> QNSETGALKTFITQQGIKSQHQTKEEQSQITSQVTGQIGWRREGIKYRRNELFLDVLESVNLLMSPQGQVLSAHVSGRVVMKSYLSGMPECKFGMNDKIVIEKQGKGTADETSKSGKQSIAIDDCTFHQCVRLSKFDSERSISFIPPDGEFELMRYRTTKDIILPFRVI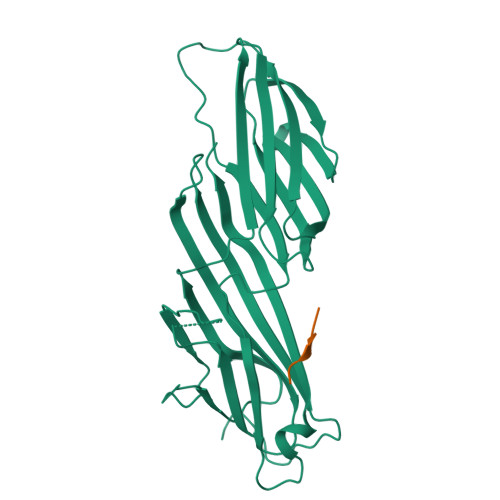PLVREVGRTKLEVKVVIKSNFKPSLLAQKIEVRIPTPLNTSGVQVICMKGKAKYKASENAIVWKIKRMAGMKESQISAEIELLPTNDKKKWARPPISMNFEVPFAPSGLKVRYLKVFEPKLNYSDHDVIKWVRYIGRSGIYETRC;> FYRALM> ADLTASFTATATLVEPARITLTYKEGAPITIMDNGNIDTELLVGTLTLGGYKTG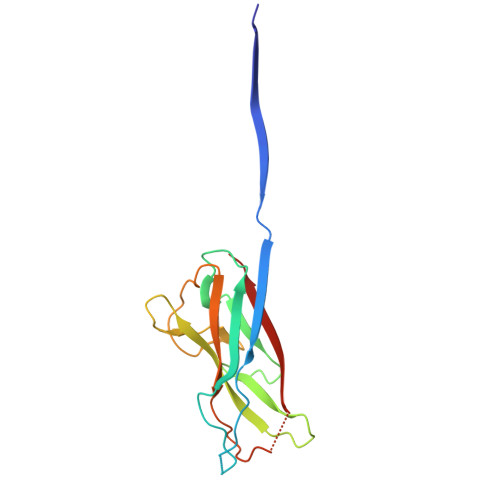TTSTSVNFTDAAGDPMYLTFTSQDGNNHQFTTKVIGKDSRDFDISPKVNGENLVGDDVVLATGSQDFFVRSIGSKGGKLAAGKYTDAVTVTVSNQ> MRGSHHHHHHGSAEPPNMPSMAPVLKNIMPAIVNVAVQGYLPNDVT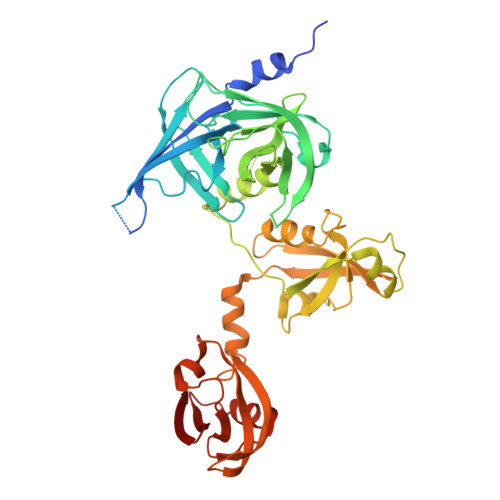PPGSAGNDEENQPNNRPPQSRMPEKGRKFESIGSGVIIDPNNGVIITNDHVIRNASLITVTLQDGRRLKARLIGGDSETDLAVLKIDAKNLKSLVIGDSDKLEVGDFVVAIGNPFGLNSFGNSQSATFGIVSALKRSDLNIEGVENFIQTDAAINPGNAGGALVNAKGELIGINTAILSPYGGNVGIGFAIPINMVKDVAQQIIKFGSIHRGLMGIFVQHLTPELAQAMGYPEDFQGALVSQVNPNSPAELAGLKAGDIITQINDTKITQATQVKTTISLLRVGSTVKIIVERDNKPLTLSAVVTDIKSHEQKLQSNNPFLYGLALRAFEQESPPHGNVIGVQVVGASENSAGWRAGIRPGDIIISANKKPVTDVKSLQTIAQEKKKELLVQVLRGPGSMYLLVI In vertebrates and some invertebrates, members of the SR gene family are hormone-activated transcription factors, which regulate developmental, reproductive, and physiological processes. The protein's ligand-binding domain (LBD) serves as an allosteric switch controlled by the hormone, which binds in an internal hydrophobic cavity deep in the protein's LBD; ligand binding shifts the domain's thermodynamic equilibrium from the inactive conformation when ligand is absent to the active conformation when ligand is bound. In the active conformation, AF-H packs against the body of the protein, contributing to the assembly of a new surface that attracts coactivator proteins that alter chromatin or otherwise potentiate transcription of nearby target genes. In contrast to vertebrate SRs, mollusks contain a single SR ortholog that is unique in being a ligand-independent constitutive transcriptional activator.

To understand the mechanisms by which constitutive activity evolved in the Crassostrea gigas ER (CgER), we used X-ray crystallography to determine the three-dimensional structure of its LBD at a resolution of 2.6 Å in the absence of any added ligands. The domain is in the classic active conformation, and the backbone conformation is similar to that of the human ERα (1.36 Å RMSD for all atoms). Unlike other SRs previously studied, there is no electron density of a ligand in the interior of the CgER LBD. Rather, the internal cavity where ligand binds in other steroid receptors is occupied in CgER by several bulky hydrophobic side-chains, including F425 and F525, and – to a lesser extent – F524 (using human ERα numbering to facilitate comparison). These hydrophobic residues would strongly clash with estradiol as it is oriented in the human ERα LBD. The resulting cavity has a total volume (168±8 Å3) much smaller than that of human ERα (402 Å3) and too small to accommodate estradiol (245 Å3) and other steroids. First, it indicates that CgER is an authentically ligand-independent transcriptional activator, which exists in the active conformation in the absence of ligand or other apparent modifications. Second, the presence in the protein interior of bulky residues that occlude the ligand cavity provides a physical rationale for the inability of mollusk ERs to bind or be activated by ligands. Examination of the CgER structure suggests that the historical substitutions confer constitutive activity not by filling the ligand cavity per se but by stabilizing the active conformation in the absence of ligand enough to remove allosteric control. Replacing leu with the much bulkier Phe fills this cavity and acts as a sort of linchpin that improves packing of these helices against each other, presumably stabilizing the active conformation and providing a structural explanation for this mutation's potentiating effect on activation by the receptor.

>[4x]SNAKSQTVTILQALNKAALPVLESHHNHGQPPTKVHLLNSLVKLAERELVHLINWAKNVPGYTDLSLSDQVHLIECCWMELLLLNCAFRSIEHGGKSLAFAPDLVLDRSSWSTVEMTEIFEQVAAVSEQMMQNHLHKDELLLLQAMVLVNAEVRRLASYNQIFNMQQSLLDAIVDTAQKYHPDNVRHVPAVLLLLTHIRQAGERGIAFFQRLKSEGVVTFCDLLKEMLDAQDFLEKKSSN> GSHMTPQLLEEQERLIATLIEAHRKTYDASYSDFSQFRPPKRGDGSPECRNATNPFLMSLLNSDMDELPKASASGAEAAAGDELSMLPHLADLVSYSIQKVIGFAKMIPGFKELCTEDQISLLKASAIEIIILRSNESFTMEDNSWTCGSNEFKYQIGDVMQAGHKLELLEPLVKFQVNMKKLDLHEAEHVLL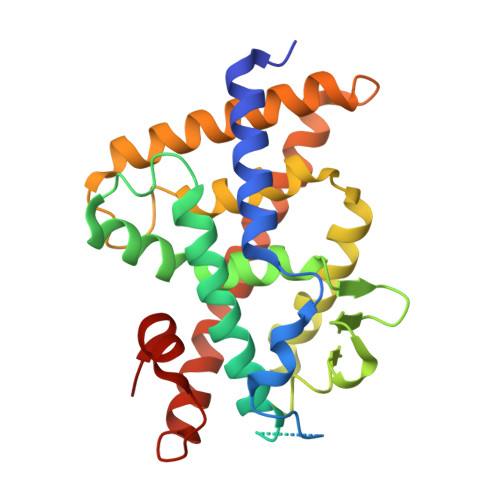MAICLFSPDRPGVQDRCRVEEVQEHLTETLRAYIACRHPLSCKHMLYTKMVEKLTELRSLNEEHSKQYLQISQDAVNKEDLPPLLLEVFGNPTA>GSAAPE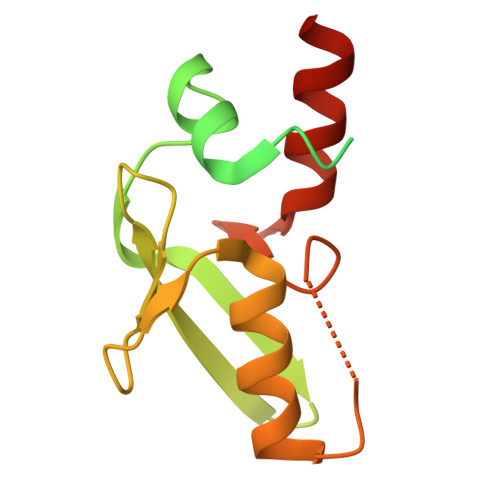SLSPGATAEEAPEEDEDDAEAEDPERGTGSGGRSGSLGGSGGGTAGPGMALGGALTRRAVTLRVLLKDELLEPGEGVLSIYYLGRKFTGDLQLDGRIVWQETGQVFNSPSAWATHCKKLVNPAKKSGCGWASVKYKGQKLDKYKAAWLRRHQLHM[2x]> GHMAEVLVVTSKVKKLIKEKGQMNTSAETIDVLSKAIEQLCLKGVESAKADGRKTVMARDIVIDHL

In this study, we present crystal structures and biochemical characterization of the free and DNA-bound forms of the histone homolog HBb from the predatory Gram-negative bacterium Bdellovibrio bacteriovorus. Our findings demonstrate that the single histone fold protein HBb forms a homodimer that has the ability to bind and bend DNA. Furthermore, we establish that HBb is essential for maintaining bacterial viability. Building on this, by employing various biophysical and biochemical approaches, we further substantiated the ability of HBb to bind and compact DNA by bending in a sequence-independent manner.

Crystallization trials were conducted with purified HBb, and within a few days, we obtained crystals that diffracted to atomic resolution. Except for the first three and last three amino acids, the full chain is clearly resolved in the electron density map. The asymmetric unit contains a single chain of HBb, forming a dimer through crystallographic symmetry. HBb exhibits a characteristic dimeric histone fold, with monomers consisting of three α-helices (α1, α2, α3) connected by two loops (l1 and l2). Dimerization occurs through the antiparallel alignment of the central α2-helices of the two monomers at an angle of approximately 25°. The dimer is stabilized primarily by hydrophobic contacts along the interface, involving residues L31, I35, and L38 in α2, as well as contributions from α1 (e.g. V11) and α3 (e.g. I59). In contrast to the archaeal histone HMfB, the α2-helix of HBb is one turn shorter, and α3 comprises only a single helical turn. Like HMfB, HBb features a conserved intramolecular salt bridge, known as the RD clamp, involving residues R51 and D58. In HBb, this motif is augmented by D49, which forms an additional salt bridge with R51, potentially stabilizing the conserved KT motif in loop l2. Four of the six DNA-binding residues in HMfB, including K52 and T53, are conserved in HBb, indicating a potential for DNA binding.>GPLGMAR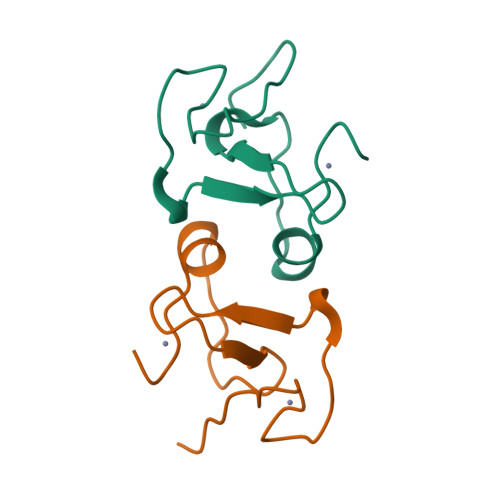DIQLPCDGDGVCMRCKSNPPPEESLTCGTCVTPWHVSCLSSPPKTLASTLQWHCPDCSGE[2x]N-{3-[(2-aminopyrimidin-5-yl)ethynyl]-2,4-difluorophenyl}-5-chloro-2-methoxypyridine-3-sulfonamide | C18 H12 Cl F2 N5 O3 S | 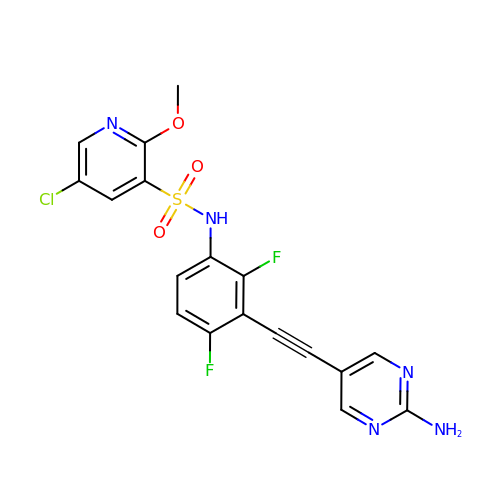JGHVXJKGYJYWOP-UHFFFAOYSA-N>[2x]CG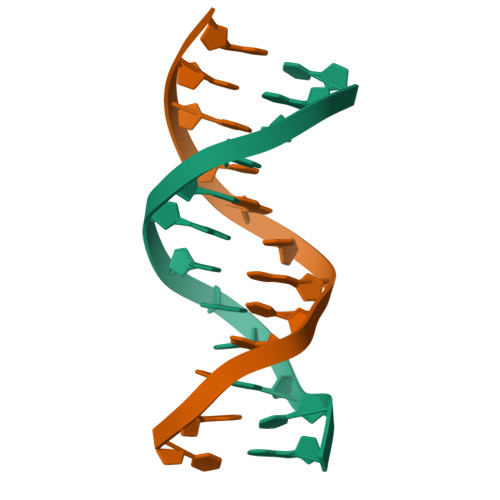CATATATGCG>[2x]GMAPPSVFAEVPQAQPVLVFKLIADFREDPDPRKVNLGVGAYRTDDCQPWVLPVVRKVEQRIANNSSLNHEYLPILGLAEFRTCASRLALGDDSPALQEKRVGGVQSLGGTGALRIGAEFLARWYNGTNNKDTPVYVSSPTWENHNGVFTTAGFKDIRSYRYWDTEKRGLDLQ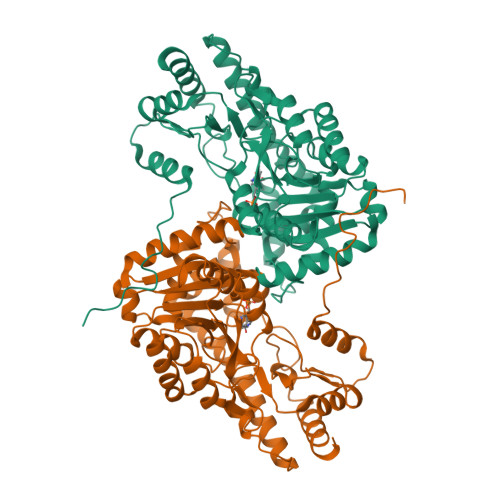GFLSDLENAPEFSIFVLHACAHNPTGTDPTPEQWKQIASVMKRRFLFPFFTSAYQGFASGNLEKDAWAIRYFVSEGFELFCAQSFSKNFGLYNERVGNLTVVAKEPDSILRVLSQMQKIVRVTWSNPPAQGARIVARTLSDPELFHEWTGNVKTMADRILSMRSELRARLEALKTPGTWNHITDQIGMFSFTGLNPKQVEYLINQKHIYLLPSGRINMCGLTTKNLDYVATSIHEAVTKIQ>[5x]SNAMIIRPEQHWFLRLFDWHGSVLSKIIFRLLLNVLMSIIAIISYQWYEQLGIHLTVAPFSLLGIAIAIFLGFRNSASYSRFVEARNLWGTVLIAERTLVRQLRNILPAEHDAHRRIVSYLVAFSWSLKHQLRKTDPTADLRRLLP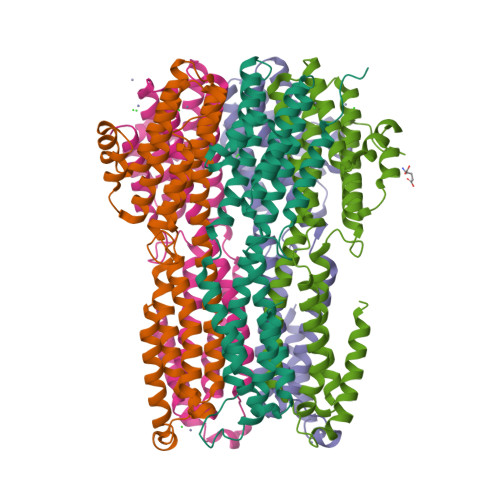EERVTEILASSMPTNRILLLAGNEIGQLREAGKLSDITYGLMDNKLDELAHVLGGCERLATTPVPFAYTLILQRTVYLFCTLLPFALVGDLHYMTPFVSVFISYTFLSWDSLAEELEDPFATAANDLPLNAMCNTIERNLLDMTGQHPLPE>[4x]TPFIRPDMKAFLEAIAAMAGPTLAEMTLEEARASYVALHGMADRPARELAVIRNLSCPGPAGDIPLRLYDARESR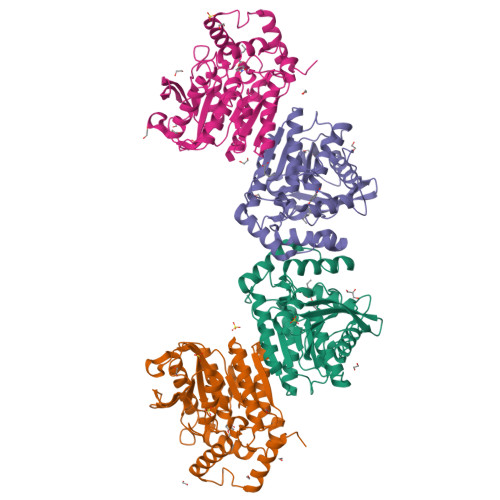EAGPVITFYHGGGFVIGDLDTHHNLCTEIAALMDLPVVAVDYRLAPEHPFPAAIEDCEAATRWVASSPSELGRTASGVIPIGDSAGGNATIVVSQLLGAKPADVPVVLQVPIFPLASDAVGSASLEAFAEGFVLTKASIEFFDTAYKADRADPRGFPILGDHTAAPPTIVATASLDPIRDSGRDYAKALVEAGRDVVYLEMEGVTHSFTNIRAAVPSTQGDLERIIAAMKMMLGTA>[3x]GPDSASR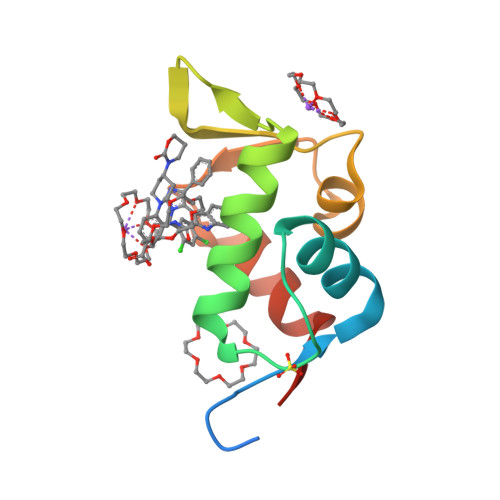ISPGQINQVRPKLPLLKILHAAGAQGEMFTVKEVMHYLGQYIMVKQLYDQQEQHMVYCGGDLLGELLGRQSFSVKDPSPLYDMLRKNLVTLAT>MRMVDIIIKKQNGKELTTEEIQFFVNGYTDGSIPDYQASALAMAIFFRDMSDRERADLTMAMVNSGETIDLSAIEGIKVDKHSTGGVGDTTTLVLAPLVAALDVPVAKMSGRGLGHTGGTIDKLEAIDGFHVELTKREFIKLVNRDKVAVIGQSGNLTPADKKLYALRDVTGTVNSIPLIASSIMSKKIAAGADAIVLDVKTGAGAFMKTEEDAAELAKAMVRIGNNVGRQTMAVISDMSQPLGFAIGNALEVKEAIDTLKGEGPEDLHELVLTLGSQMVVLAKKADTLDEARAKLEEVMKNGKALEKFKDFLKNQGGDSSIVDDPSKLPQAAYQIDVPAKEAGVVSEIVADEIGVAAMLLGAGRA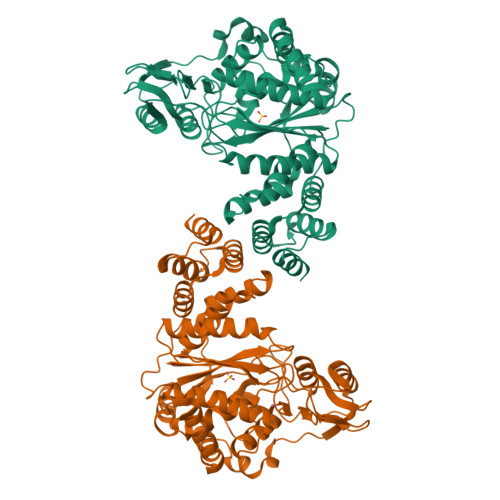TKEDEIDLAVGIMLRKKVGDKVEKGEPLVTLYANRENVDEVIAKVYDNIRIAAEAKAPKLIHTLITE[2x]> MEGRFREFQQGNECQIDRLTALEPTNRIQAERGLTEVWDSNEQEFRCAGVSVIRRTIEPHGLLLPSFTSAPELIYIEQGNGITGMMIPGCPE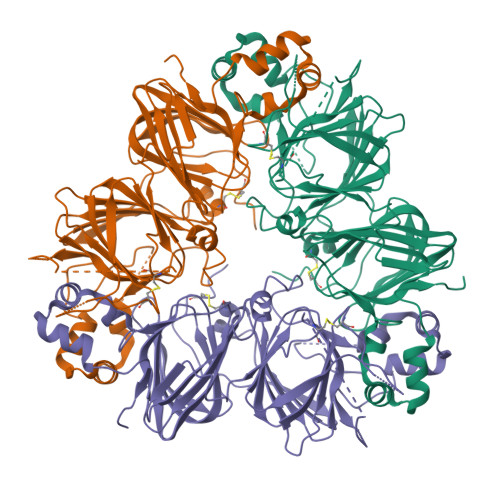TYESGSQQFQGGEDERIREQGSRKFGMRGDRFQDQHQKIRHLREGDIFAMPAGVSHWAYNNGDQPLVAVILIDTANHANQLDKNFPTRFYLAGKPQQEHSGEHQFSRESRRGERNTGNIFRGFETRLLAESFGVSEEIAQKLQAEQDDRGNIVRVQEGLHVIKPPSRAWEEREQGSRGSRYLPNGVEETICSARLAVNVDDPSKADVYTPEAGRLTTVNSFNLPILRHLRLSAAKGVLYRNAMMAPHYNLNAHNIMYCVRGRGRIQIVNDQGQSVFDEELSRGQLVVVPQNFAIVKQAFEDGFEWVSFKTSENAMFQSLAGRTSAIRSLPIDVVSNIYQISREEAFGLKFNRPETTLFRSSGQGEYRRKISIA~{N}-(4-chlorophenyl)-2-phenylmethoxy-ethanamide | C15 H14 Cl N O2 | 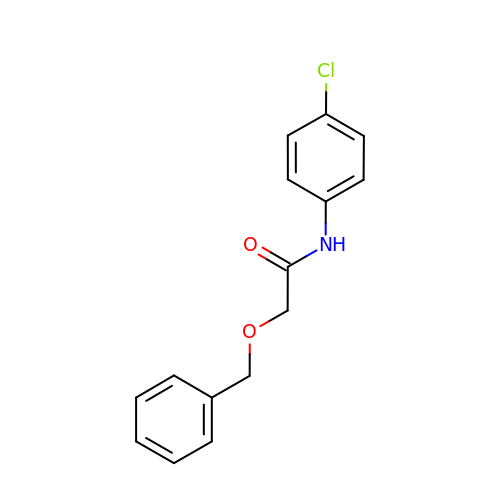CELZHXIAORJPBI-UHFFFAOYSA-N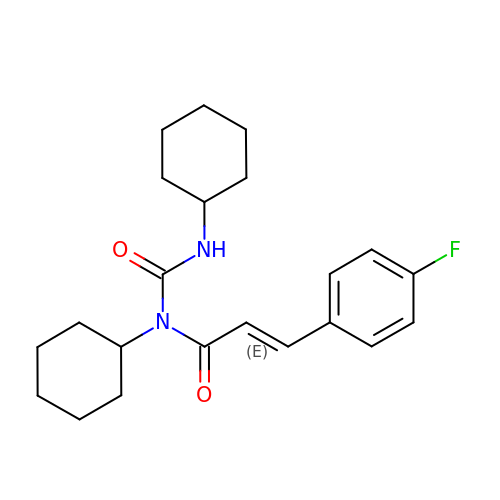(2E)-N-cyclohexyl-N-(cyclohexylcarbamoyl)-3-(4-fluorophenyl)prop-2-enamide | C22 H29 F N2 O2 | GUDFNCYAKAJWRN-DTQAZKPQSA-N> TTIVSVRRNGHVVIAGDGQATLGNTVMKGNVKKVRRLYNDKVIAGFAGGTADAFTLFELFERKLEMHQGHLVKAAVELAKDWRTDRMLRKLEALL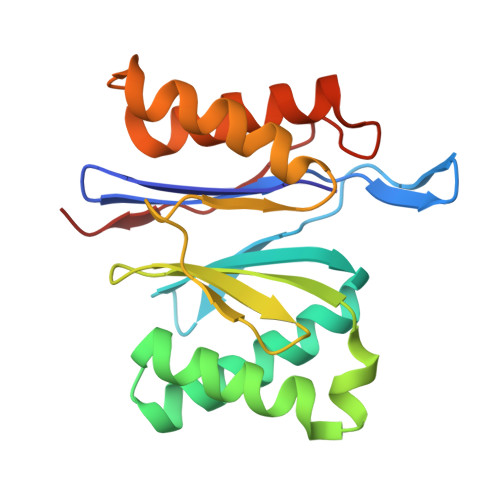AVADETASLIITGNGDVVQPENDLIAIGSGGPYAQAAARALLENTELSAREIAEKALDIAGDICIYTNHFHTIEELSYK>[4x]GASRQRKLEALIRDPRSPINVESLLDGLNSLVLDLDFPALRKNKNIDNFLNRYEKIVKKIRGLQMKAEDYDVVKVIGRGAFGEVQLVRHKASQKVY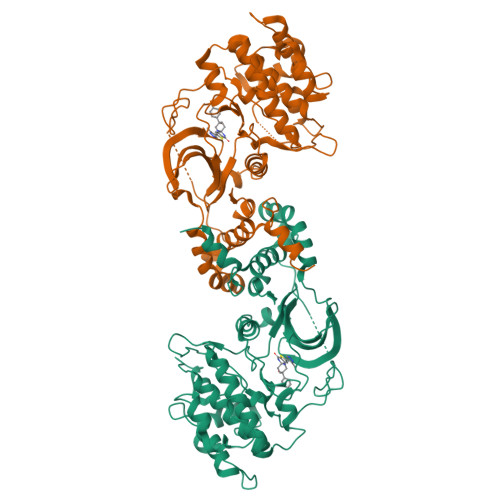AMKLLSKFEMIKRSDSAFFWEERDIMAFANSPWVVQLFYAFQDDRYLYMVMEYMPGGDLVNLMSNYDVPEKWAKFYTAEVVLALDAIHSMGLIHRDVKPDNMLLDKHGHLKLADFGTCMKMDETGMVHCDTAVGTPDYISPEVLKSQGGDGYYGRECDWWSVGVFLYEMLVGDTPFYADSLVGTYSKIMDHKNSLCFPEDAEISKHAKNLICAFLTDREVRLGRNGVEEIRQHPFFKNDQWHWDNIRETAAPVVPELSSDIDSSNFDDIEDDKGDVETFPIPKAFVGNQLPFIGFTYYR(2S)-3-cyclohexyl-2-(6-fluoro-2,4-dioxo-1,4-dihydroquinazolin-3(2H)-yl)-N-(1,3-thiazol-2-yl)propanamide | C20 H21 F 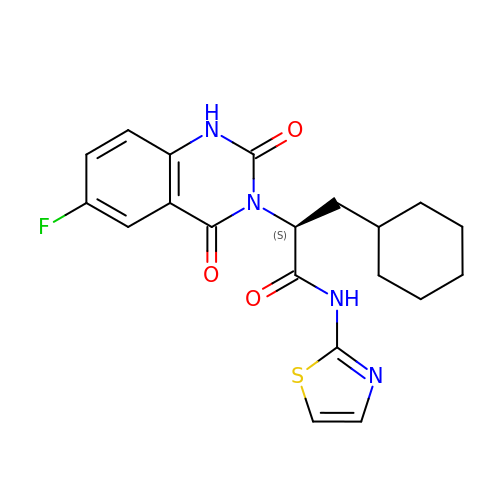N4 O3 S | FWNYYSSFAUKKJU-INIZCTEOSA-N MnmE is an evolutionary conserved G protein found in bacteria, fungi, and humans, which together with the protein GidA catalyzes the formation of a carboxymethylaminomethyl-group (cmnm) at the 5 position of the wobble uridine (U34) of tRNAs reading 2-fold degenerated codons ending with A or G, i.e., tRNAArg(UCU), tRNAGln(UUG), tRNAGlu(UUC), tRNALeu(UAA), and tRNALys(UUU). The crystal structure of MnmE from Thermotoga maritima reveals a three-domain protein consisting of an N-terminal tetrahydrofolate-binding domain, a central helical domain, and a canonical Ras-like G domain inserted into the helical domain. On the basis of the common feature that the G domain cycle is regulated by homodimerization, MnmE has been categorized as G protein activated by nucleotide-dependent dimerization (GAD), together with the signal recognition particle (SRP) and its receptor (SR), the regulator of Ni insertion into hydrogenases HypB, the dynamins, the human guanylate binding protein hGBP1, the chloroplast import receptors Toc33/34, the septins, and the Roc-COR tandem found to be mutated in Parkinson disease. The X-ray structures show MnmE to be a constitutive homodimer where the highly mobile G domains face each other in various orientations but are not in close contact as suggested by the GDP-AlFx structure of the isolated domains.

NoMnmE crystals with sufficient diffraction were obtained in a PEG 550 monomethyl ether (MME) condition. CtMnmE·GDP and NoMnmE·GDP (grown in presence of AlFx) crystallized in the space groups I4(1)22 and P4(3)2(1)2, respectively, each with one full length protomer in the asymmetric unit. In both cases homodimers are formed via crystallographic symmetry by means of the N-terminal domains. Strikingly, two molecules of 5-formyl-tetrahydrofolate (5-F-THF) were identified in the structure of NoMnmE·GDP, which were apparently copurified from the bacterial expression system. This suggests a high affinity for 5-F-THF and supports the recently proposed enzymatic mechanism whereby the C1 group of the cmnm modification is donated by THF. In NoMnmE·GDP, two Zn2+ atoms from the crystallisation condition, localized by their anomalous signal, are coordinated to the G domain. One of these is coordinated to helix Gα4 and is involved in crystal contacts (see below), the other occupies the usual Mg2+-binding site at the β-phosphate of GDP. As Switch I is resolved, but does not contact the bound GDP and since there is no indication for a physiological role of Zn2+, we consider this to be a crystallographic artefact also observed in the nucleotide binding pockets of other small G proteins. In NoMnmE·GDP a Zn2+-ion tightly links the G domain to symmetry mates, while in CtMnmE·GDP the G domains fix each other by a toothing upside-down arrangement.

> GSHMAITGTIAAIATAIVPQQGSVGIVRVSGSQAIAIAQTLFDAPGKQVWESHRILYGYIRHPQTRQIVDEALLLLMKAPRSYTREDVVEFHCHGGIIAVQQVLQLCLESGARLAQPGEFTLRAFLNGRLDLTQAESIADLVGARSPQAAQTALAGLQGKLAHPIRQLRANCLDILAEIEARIDFEEDLPPLDDEAIISDIENIAAEISQLLATKDKGELLRTGLKVAIVGRPNVGKSSLLNAWSQSDRAIVTDLPGTTRDVVESQLVVGGIPVQVLDTAGIRETSDQVEKIGVERSRQAANTADLVLLTIDAATGWTTGDQEIYEQVKHRPLILVMNKIDLVEKQLITSLEYPENITQIVHTAAAQKQGIDSLETAILEIVQTGKVQAADMDLAINQRQAAALTQAKMSLEQVQATITQQLPLDFWTIDLRGAIQALGEITGEEVTESVLDRIFSRFCIGK> MMIIVGVDAGGTKTKAVAYDCEGNFIGEGSSGP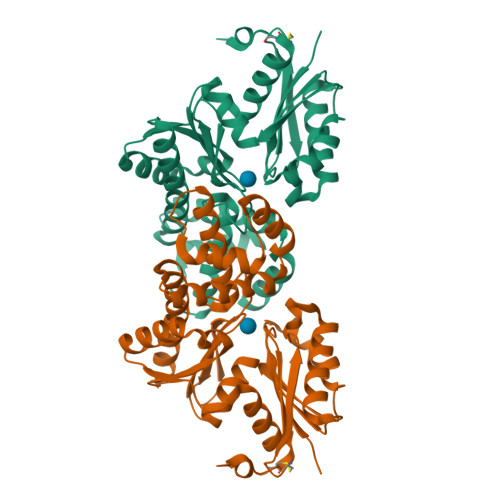GNYHNVGLTRAIENIKEAVKIAAKGEADVVGMGVAGLDSKFDWENFTPLASLIAPKVIIQHDGVIALFAETLGEPGVVVIAGTGSVVEGYNGKEFLRVGGRGWLLSDDGSAYWVGRKALRKVLKMMDGLENKTILYNKVLKTINVKDLDELVMWSYTSSCQIDLVASIAKAVDEAANEGDTVAMDILKQGAELLASQAVYLARKIGTNKVYLKGGMFRSNIYHKFFTLYLEKEGIISDLGKRSPEIGAVILAYKEVGCDIKKLISD> AQGMIICNNQIDDDQLKAIQDLASLCREHDGGTPTFYNHLLIQKRPTENNVLYFQDNQLLGFLSVYFFYEDACEVSLIVSPLHRRQGIAKQLLQTIMPLLTAKEMTTLIFSTPTEINDDWLINQGFSYRNSEYHMQRNGYDPIFMPTPKLHIRKATEDDIP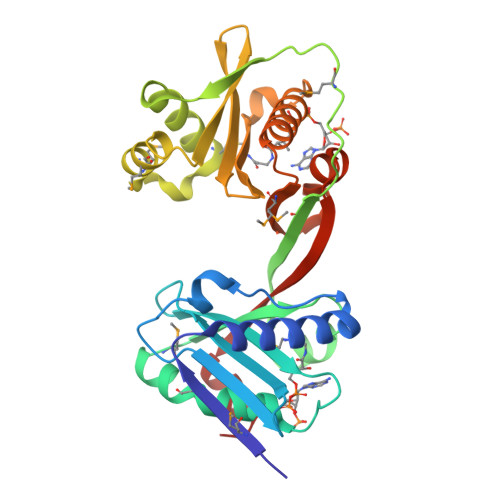ALCAIDEACFPEHQENMISRFSMLLNDASYTLFLASYNHIIVGKAHIHWQSKEAIFSDIAIFPQYQGQGWGGELLSYCINQALTSGKNKLMLDVETSNQNALHLYTRLGFKTANVSDYWVIPLPQLLTNWALE> GAMVAAQKKKAQDEYGAASITILEGLEAVRKRPGMYIGSTGERGLHHLIWEVVDNAVDEAMAGYATTVNVVLLEDGGVEVADDGRGIPVATHASGIPTVDVVMTQLHAGGKFDSDAYAISGGLHGVGVSVVNALSTRLEVEIKRDGYEWSQVYEKSEPLGLKQGAPTKKTGSTVRFWADPAVFETTEYDFETVARRLQEMAFLNKGLTINLTDERVTQDEVVDEVVSDVAEAPKSASERAAESTAPHKVKSRTFHYPGGLVDFVKHINRTKNAIHSSIVDFSGKGTGHEVEIAMQ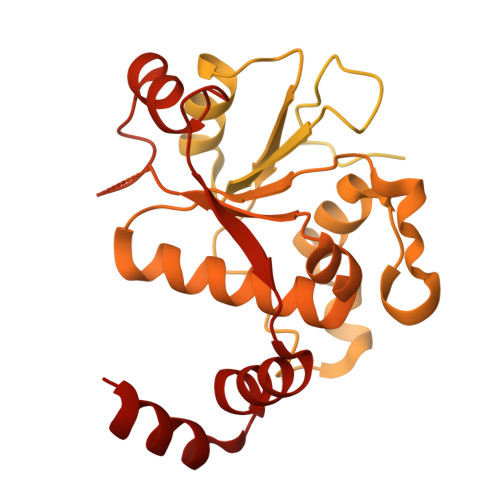WNAGYSESVHTFANTINTHEGGTHEEGFRSALTSVVNKYAKDRKLLKDKDPNLTGDDIREGLAAVISVKVSEPQFEGQTKTKLGNTEVKSFVQKVCNEQLTHWFEANPTDAKVVVNKAVSSAQARIAARKARELVRRKSATDIGGLPGKLADCRSTDPRKSELYVVEGDSAGGSAKSGRDSMFQAILPLRGKIINVEKARIDRVLKNTEVQAIITALGTGIHDEFDIGKLRYHKIVLMADADVDGQHISTLLLTLLFRFMRPLIENGHVFLAQPPLYKLKWQRSDPEFAYSDRERDGLLEAGLKAGKKINKEDGIQRYKGLGEMDAKELWETTMDPSVRVLRQVTLDDAAAADELFSILMGEDVDARRSFITRNAKDVRFLDV>MLYEEDYKLALEAFKKVFNALTHYGAKQAFRSRARDLVEEIYNSGFIPTFFYIISKAELNSDSLDSLISLFSSDNAILRGSDENVSYSAYLFIILYYLIKRGIIEQKFLIQALRCEKTRLDLIDKLYNLAPIISAKIRTYLLAIKRLSEALIEAR[3x];>[4x]MPYYAFAEPFFIHAITHLHVGSGSSVEEEIALPFQRDELGYPTIYASSLKGAIKSFLLKEFPDKRDVIYKVLGEDENPEEASLGTFLDAILFAIPSRIIEIDSAKPYVWVYVTTYELLKKVKLYLDSISQLSNASFSNLKNKIDTILAKEGKNITLDSDLKSAILNEDFYVELEALNNKIPSIINAGVPLLVLEDSIGREVINRSLIRVRRIRIDRDKKVVETGGLWSEEYVPMKTIFFSVLLGKESKESAIFASCILRNLRYVILGGKETIGKGIVELRWVKDVI;> MKRVLIKPLEPLMFRSQGEFEPLITGSHTAAQSLIIPRPSTIAGMLGYILFNKSSGTGDWLSDLTNLLATIYGTFIETNGEYLFPLRMGNHLALVDQQHLINLPTLLEKEYERREKGIYELFYDKNKLFQIINHQDRIGISIDKSTRTVKEHYLYSARYLAFKKEVNYVIFIDNDAISDKINGKIVNFGGENRIAKLEVDDYKVDTSIEEEYYLALSPILIPDEALDNFLDNISDYVAMGKVDKISLGFDIANTKRKEMLTAILEGSIVKRSIIDFIKNEIKNDLRYRFSKYEKIGYNTLMSLCKLALRKILS;> MAIDFLVNILELIKEKQCNINLFSAISLTSIVYNNFGEFLSNNQSYSTNNPLLKYHIIILNDKNKTKDVEEKRNIFKREVA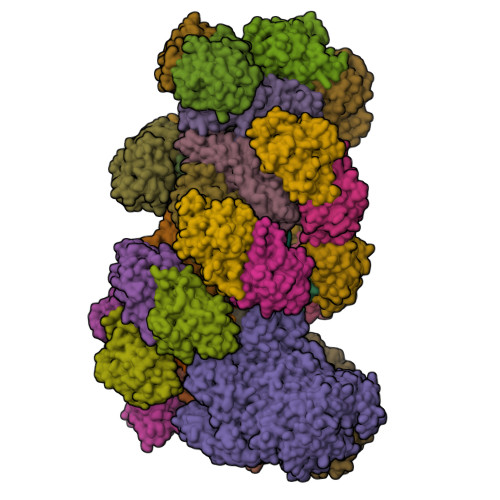ELISRNFKLDGEKVRNYFDSLKEVLKSLKYTIVDVEITTRTRALIGVSTSLGKLIFGSGISFDPYMNLPYIPASEIKGIVRSYIEGKLGEQEAEEIFGNEEREGNVNFTDAYPTRSKDFLFVPDVITPHYNGKKSEADAEPRPVIHLTIAPKVTFRFLIYYKREDVGKPICDSMPIILIRGLGARSSVGYSLFELRKIEVIKAAAHHHHHHHHHH;> MEELLMSLKLKALYPLTGGYNRHSINPFYEELVRPTEIKGLWRWWNRVLFNTLAYSTKGKLYTYESIDRLFEDVFGSENKKSAVRLEVITDEGNDNRFELSYVELDKVIDCLRNYKRKVSLDFIDNTLIAEIEGSTKIPISFKSNLDIDKIIKDLVHNNKLLSFELLGFKSVEIDATKISDKKILKEILRDLITNYLEYFNIKQEVTFTLNIYLDKSREHKQNFEDKLKFALYSLLVFILLGGIGRKTSRGFGSLSIIDVKCYDNSICKKIEDLAKNFLKISSGNELKSKIESILDCIKNSCIDTLYIENNILSEIDPKKNVVYFINSDLFEVKRINDKEKVLANIYKAVSSEGCCIKSIITDKYVRKSFLIAFGGYRKVEKDKGLDIGFIKNYLCETCETVSSFNIVDFLLSEGSFMSDYILQYEHRNSLLRFKLISDNSNNSYLIGYILHSSYFKKIDIKYVRCILEKLTYCVI;> MSIDNVLREFLDYKIIALLHDPPNKAWVITGRARNLTQQLSNIRASRKHEKVAKYIINQLFGKNYSEKVDNADKLASSIDRYLGSIVYKERSLFENRSIFLKNILLSNIQRDIGNLFPKDKSKLDNLILEYKKLLNVINKTNLILKYQLFYLIYELVWIDSKYENTPSDTRNPTHTIFDHLYATAAMMNWILSLEKEAKGYLLGIDTIGVADFISKGRKTRDLWISSYLVSALLWYVITWFIEEYGPDVILFPSLRFNQFYAFYLLEKLRKEGVSEDVIDEIKELITKYIFNGDDLFENLKIPPYPIIPGRITLILPGLIREGEEYKKVQDDNCFISKVKERYNEGWRKLIEGLRCYSERKREDGFWNLVCRVLKLTEDLLQTTPLNIRVKQVSVTEDEIFNNNKLRSDSWKIYDNKYRQLVSEFKKSKLVKVTPESRLKLFELTKFDKLPQIGEKSKRGYEFCTSCGVLPAVVIMPKEDELEKKLIDLGIARDEKDVRSIKNMISPGERLCPWCLVKRALGAEPRLMRILLLGDLYSVEKIVNEIVSRDVKIEIPSTSDIASIKTFEEMIEKKNEICEDLKEEEVCEKPSESVLSMWQWFNKNYYNGINLTIDPEEYWFSEKRRRYYFSVFRRHRITFPSPYYALVRADSDYLGDLLEGKLTPYLAGIIDSGDYANISEKKEEVNKLLEEYLVNAGSGSIVDYVKTVLKCIRENLNKCSCAEKIYSNEVAKVMFRVNVEKANVEEEVKNSLEYFETILNEGRIIVTPAWHVSISSALNRGLLVELELVNKHKGFVIYAGGDDLLAMLPVDEVLDFIKESRRAFAGFGTEKLGNMCLENGFVRINNAYYPSLPIVGRSYSVIIAHYADPLFFVINDSYNLLEEGKEIIRYRVMYNGEYKDAKKDVAIFRYQGLTSVIPLSLKRPIVSSVSDFNEIASIIDVILELKKRIDEGRISVSLLYDYEKYKHLIVASDEKYLTEFLVKDWIKRNSLRKHVEFTIDEKLYGVRLTIENYPIKIPNDLISNIVYTLRIIYGGEK;>MSTQREYVFIPITNSITIDVKITIGGSDHITNIDERGIHNVLVITGYAVDEKNGRLVPTLDPCDYVKGILVAGTPQQAQSNDFLTLKLPANKLYLIRKKGNISDDLKIYIPYSSPDARNSMKTKPVSISDDTIVNNIIKEVFDKIYNITQKEKVKIEKVKEDIKELFSYYALEQ[22x]>[2x]MLVVGSELQSDAQQLSAEAPRHGELQYLRQVEHILRCGFKKEDRTGTGTLSVFGMQARYSLRDEFPLLTTKRVFWKGVLEELLWFIKGSTNAKELSSKGVRIWDANGSRDFLDSLGFSARQEGDLGPVYGFQWRHFGAEYKDMDSDYSGQGVDQLQKVIDTIKTNPDDRRIIMCAWNPKDLPLMALPPCHALCQFYVVNGELSCQLYQRSGDMGLGVPFNIASYALLTYMIAHITGLQPGDFVHTLGDAHIYLNHIEPLKIQLQREPRPFPKLKILRKVETIDDFKVEDFQIEGYNPHPTIKMEMAV

Thymidylate synthase (EC 2.1.1.45) catalyzes the dUMP methylation reaction, involving N5,10-methylenetetrahydrofolate (meTHF)-aided concerted transfer and reduction of the one-carbon group, its products being thymidylate and dihydrofolate (DHF). N4-hydroxy-2′-deoxycytidine 5′-monophosphate (N4-OH-dCMP) is a substrate analog, reported to inhibit the enzyme from bacterial, avian and mammalian sources, as well as from certain helminths. Inhibition was found to be competitive with respect to dUMP, and apparently mechanism-based, as it showed meTHF- and time-dependence; the dependence on time pointed to the slow-binding inhibition. Novel evidence is presented allowing further clarification of the mechanism of the slow-binding thymidylate synthase (TS) inhibition by N4-hydroxy-dCMP (N4-OH-dCMP).

The crystal structure of the mouse TS-N4-OH-dCMP complex soaked with N5,10-methylenetetrahydrofolate revealed the reaction to run via a unique imidazolidine ring opening, leaving the one-carbon group bound to the N(10) atom, thus too distant from the pyrimidine C(5) atom to enable the electrophilic attack and methylene group transfer. The structure of mTS-N4-OH-dCMP complex soaked with meTHF was obtained by soaking crystals of the initial complex with approximately 50 mM solution of meTHF for a few hours. Electron density corresponding to the inhibitor and the cofactor is clearly defined in both subunits. The folate derivative is modeled with 0.88 and 0.85 occupancies for subunits A and B, respectively. The N4-OH-dCMP molecules are situated too far away from Cys189 to form covalent bonds (the distances are 3.07 Å and 2.95 Å in subunits A and B, respectively). In particular, the resolution is insufficient to unequivocally judge the oxidation levels of the pteridine ring and one-carbon group of the folate derivative (PDB ligand code: TGQ), even if scrutinized electron density maps allow leaning towards tetrahydrofolate (with the pteridine ring C(6) sp3 hybridization) and methylene group (suggested as one resulting from the imidazolidine ring opening), respectively. Of note, however, is the fact that the cofactor molecule is present in a modified form, with electron density next to the N(10) atom, suggesting the one-carbon group to be covalently bound to N(10) instead N(5). Thus the imidazolidine ring must have been apparently opened in an unusual manner, on the N(5) rather than N(10) side. Analysis of residues remaining in a close proximity to TGQ shows that the one-carbon group is orientated toward the inhibitor N(4) atom, separated from it by the distances of 3.43 Å and 3.34 Å in the subunits A and B, respectively. Thus, with N4-OH-dCMP bound in the active site the imidazolidine ring opens at the N(5) site, in a striking contrast to the corresponding phenomenon observed with dUMP and FdUMP, the difference resulting apparently from the presence of the N4-OH residue.> MTKFSGNELRAELYRRAFLSYSVAPGALGMFGRSLLAKGARAEALANGTVMSGSHWGVFTATVENGRATAFTPWEKDPHPSPMLAGVLDSIYSPTRIKYPMVRREFLEKGVNADRSTRGNGDFVRVSWDQALDLVAAEVKRVEETYGPEGVFGGSYGWKSPGRLHNCTTLLRRMLTLAGGYVNGAGDYSTGAAQVIMPHVVGTLEVYEQQTAWPVLAENTEVMVFWAADPIKTSQIGWVIPEHGAYPGLEALKAKGTKVIVIDPVRTKTVEFFGAEHITPKPQTDVAIMLGMAHTLVAEDLYDKDFIANYTSGFDKFLPYLDGETDSTPKTAEWAEGISGVPAETIKELARLFESKRTMLAAGWSMQRMHHGEQAHWMLVTLASMLGQIGLPGGGFGLSYHYSGGGTPSTSGPALAGITDGGAATKGPEWLAASGASVIPVARVVDMLENPGAEFDFNGTRSKFPDVKMAYWVGGNPF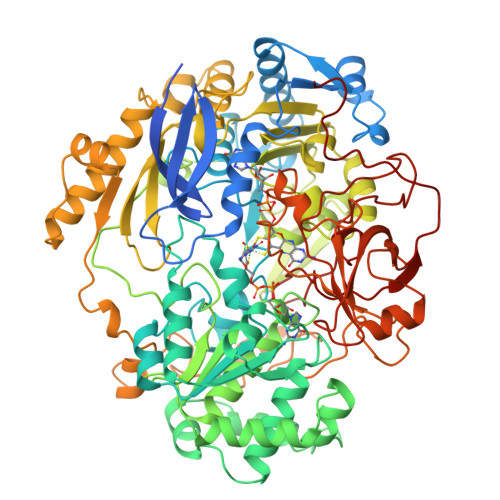VHHQDRNRMVKAWEKLETFVVHDFQWTPTARHADIVLPATTSYERNDIETIGDYSNTGILAMKKIVEPLYEARSDYDIFAAVAERLGKGAEFTEGKDEMGWIKSFYDDAAKQGKAAGVQMPAFDAFWAEGIVEFPVTDGADFVRYASFREDPLLNPLGTPTGLIEIYSKNIEKMGYDDCPAHPTWMEPLERLDGPGAKYPLHIAASHPFNRLHSQLNGTVLREGYAVQGHEPCLMHPDDAAARGIADGDVVRVHNDRGQILTGVKVTDAVMKGVIQIYEGGWYDPSDVTEPGTLDKYGDVNVLSADIGTSKLAQGNCGQTVLAEVEKYTGPAVTLTGFVAPKAAE>[4x]MAIDLRPFIPFGRGALSQATDPFRAAVEFTLMPMLITNPHLPDNPIVFANPAFLKLTGYEADEVMGRNCRFLQGHGTDPAHVRAIKSAIAAEKPIDIDIINYKKSGEAFWNRLHISPVHNANGRLQHFVSSQLDVTLELSRLVELEKERKTLSIETARSKDQLDYIVEVANIGFWTREFYSGKMTCSAECRRIYGFTPDEPVH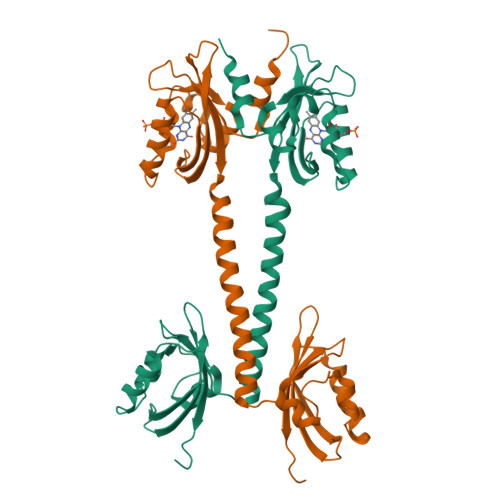FDTILDLVVLEDRMTVVQKAHQAVTGEPYSIEYRIVTRLGETRWLETRAKALTGENPLVLGIVQDVTERKHHHHHH> MEFYDSDVVVVGAGPTGLMLAGELRLAGVSVVVLDKLAEPIKESRALGFSARTIEEFAQRGLMDRFGEVGVIPVGHFGGVPLDYQVIEGGSYGARGIPQARTEGILGGWARELGAEVRRGYEVTAIEDTGTSVTVEAAGADGSPLSLRARYVVGCDGARSSVRKLAGIDFPGTEPAIELRFADVAGVQLRPRFSGERVPGGMVMVLPMGPDRCRVIYFDSSQPLRTAPEAITFEEVADSWQRLTGEDISGATPLWVSSATDVSRQAAQYRKGRVFLAGDAAHIHLPIGAQGMSAGVQDAVNLGW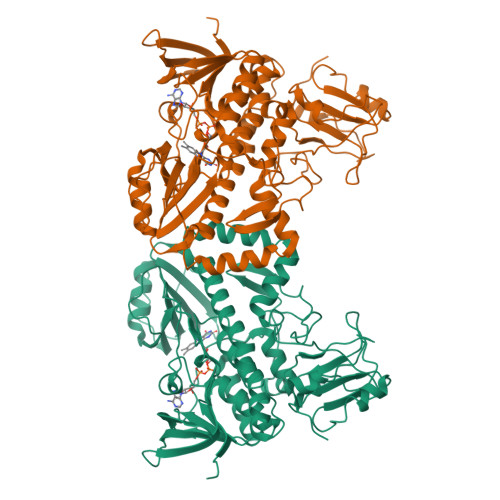KLALDISGRAPQGLLDTYHSERHPVGQRILTNTLAQRILYLGGDEITPMREVLAELMGSHVSVQRHLAGMVTGLDIRHDVGEGDHPLLGRRLPDRELVVDGEKIPFYSLLRPGRAVLLELGGDRGLRTAAAGWADRVDLVAAEFDGCEAPVDGILVRPDGYVAWVAALGAGADGLTTALDRWFGPTA> GGACAGAGUAGGUAAACGUGCGUAAAGUGCCUGAGGGACGGGGAGUU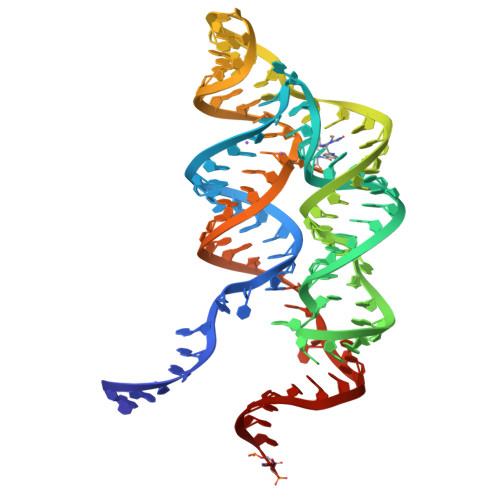GUCCUCAGGACGAACACCGAAAGGUGGCGGUACGUUUACCGCAUCUCGCUGUUC>[4x]GSDEAAELMQQVNVLKLTVEDLEKERDFYFGKLRNIELICQENEGENDPVLQRIV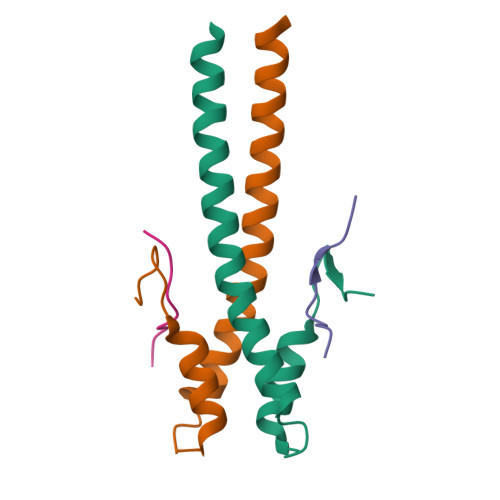DILYATDEGFVIPDEGG;>GSRPSTAKPSKIPTPQRKSPASKLDKSSKR[4x]>MKYMIPDEEFIRREGVPITKEEIRAVSIGKLNLNKDDVVVDVGCGSGGMTVEIAKRCKFVYAIDYLDGAIEVTKQNLAKFNIKNCQIIKGRAEDVLDKLEFNKAFIGGTKNIEKIIEILDKKKINHIVANTIVLENAAKIINEFE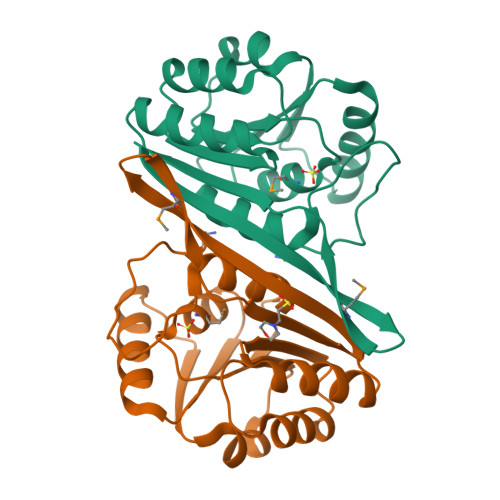SRGYNVDAVNVFISYAKKIPSGHMFLAKNPITIIKAVR[2x]>HHHHHHMSVTTPRRETSLLSRALRATAAAATAVVATVALAAPAQAANPYERGPNPTESMLEARSGPFSVSEERASRFGADGFGGGTIYYPRENNTYGAIAISPGYTGTQSSIAWLGERIASHGFVVIAIDTNTTLDQPDSRARQLNAALDYMLTDASSAVRNRIDASRLAVMGHSMGGGGTLRLASQRPDLKAAIPLTPWHLNKSWRDITVPTLIIGAEYDTIASVTLHSKPFYNSIPSPTDKAYLELDGASHFAPNITNKTIGMYS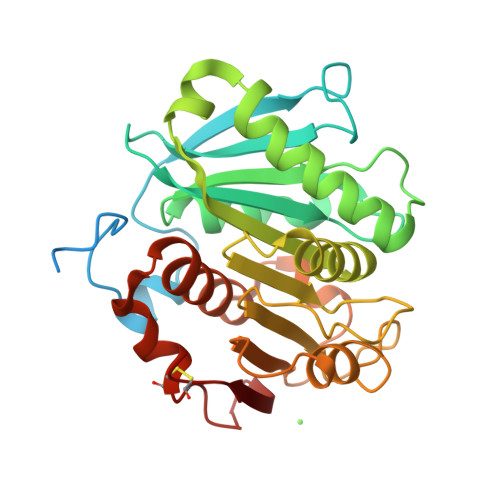VAWLKRFVDEDTRYTQFLCPGPRTGLLSDVEEYRSTCPF[2x]> APLVHHHHHHALDENLYFQGALADVSRPPHARKTGGSSPETKYDQPPKCDISGKEA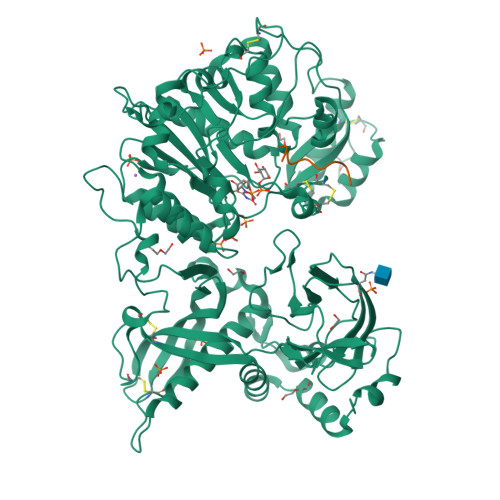ISALSRAKSKHCRQEIGETYCRHKLGLLMPEKVTRFCPLEGKANKNVQWDEDSVEYMPANPVRIAFVLVVHGRASRQLQRMFKAIYHKDHFYYIHVDKRSNYLHRQVLQVSRQYSNVRVTPWRMATIWGGASLLSTYLQSMRDLLEMTDWPWDFFINLSAADYPIRTNDQLVAFLSRYRDMNFLKSHGRDNARFIRKQGLDRLFLECDAHMWRLGDRRIPEGIAVDGGSDWFLLNRRFVEYVTFSTDDLVTKMKQFYSYTLLPAESFFHTVLENSPHCDTMVDNNLRITNWNRKLGCKCQYKHIVDWCGCSPNDFKPQDFHRFQQTARPTFFARKFEAVVNQEIIGQLDYYLYGNYPAGTPGLRSYWENVYDEPDGIHSLSDVTLTLYHSFARLGLRRAETSLHTDGENSCRYYPMGHPASVHLYFLADRFQGFLIKHHATNLAVSKLETLETWVMPKKVFKIASPPSDFGRLQFSEVGTDWDAKERLFRNFGGLLGPMDEPVGMQKWGKGPNVTVTVIWVDPVNVIAATYDILIESTAEFTHYKPPLNLPLRPGVWTVKILHHWVPVAETKFLVAPLTFSNRQPIKPEEALKLHNGPLRNAYMEQSFQSLNPVLSLPINPAQVEQARRNAASTGTALEGWLDSLVGGMWTAMDICATGPTACPVMQTCSQTAWSSFSPDPKSELGAVKPDGRLR;> QEEEGAGGGQGG>SMPQSKSRKIAILGYRSVGKSSLTIQFVEGQFVDSYDPTIENTFTKLITVNGQEYHLQLVDTAGQDEYSIFPQTYSIDINGYILVYSVTSIK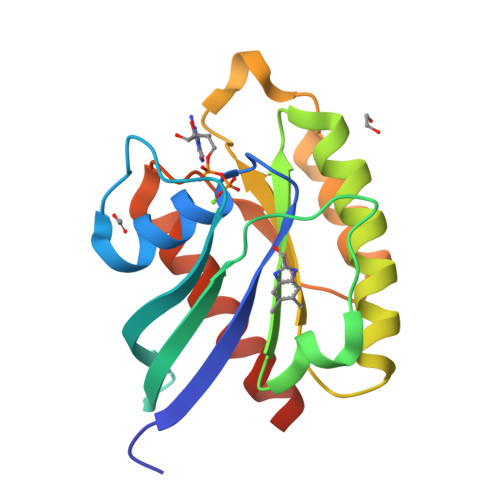SFEVIKVIHGKLLDMVGKVQIPIMLVGNKKDLHMERVISYEEGKALAESWNAAFLESSAKENQTAVDVFRRIILEAEKLEHHHHHH[4x]>MSDYFEEVMRKLTIEDVSILGWLFQNEANAVFKAIKKSSIADELEYSTANFRKTLNKLEAIHFIGTVTGGKEHKLYLTEYGQQAVQQAIHHGE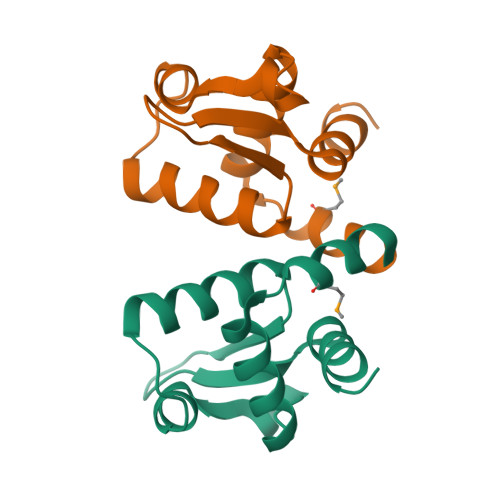ENEEVEEI[3x]>[2x]MRRETVGEFSSDDDDDILLELGTRPPRFTQIPPSSAALQTQIPTTLEVTTTTLNNKQSKNDNQLVNQLNKAQGEASMLRDKINFLNIEREKEKNIQAVKVNELQVKHLQELAKLKQELQKLEDEKKFLQMEARGKSKREVITNVKPPSTTLSTNTNTITPDSSSVAIEAKPQSPQSKKRKISDNLLKKNMVPLNPNRIIPDETSLFLESILLHQIIGADLSTIEILNRLKLDYITEFKFKNFVIAKGAPIGKSIVSLLLRCKKTLTLDRFIDTLLEDIAVLIKEISVHPNESKLAVPFLVALMYQIVQFRPSATHNLALKDCFLFICDLIRIYHHVLKVPIHESNMNLHVEPQIFQYELIDYLIISYSFDLLEGILRVLQSHPKQTYMEFFDENILKSFEFVYKLALTISYKPMVNVIFSAVEVVNIITSIILNMDNSSDLKSLISGSWWRDCITRLYALLEKEIKSGDVYNENVDTTTLHMSKYHDFFGLIRNIGDNELGGLISKLIYTDRLQSVPRVISKEDIGMDSDKFTAPIIGYKMEKWLLKLKDEVLNIFENLLMIYGDDATIVNGEMLIHSSKFLSREQALMIERYVGQDSPNLDLRCHLIEHTLTIIYRLWKDHFKQLREEQIKQVESQLIMSLWRFLVCQTETVTANEREMRDHRHLVDSLHDLTIKDQASYYEDAFEDLPEYIEEELKMQLNKRTGRIMQVKYDEKFQEMARTILESKSFDLTTLEEADSLYISMGL;>[2x]MESHVKYLDELILAIKDLNSGVDSKVQIKKVPTDPSSSQEYAKSLKILNTLIRNLKDQRRNNIMKNDTIFSKTVSALALLLEYNPFLLVMKDSNGNFEIQRLIDDFLNISVLNYDNYHRIWFMRRKLGSWCKACVEFYGKPAKFQLTAHFENTMNLYEQALTEVLLGKTELLKFYDTLKGLYILLYWFTSEYSTFGNSIAFLDSSLGFTKFDFNFQRLIRIVLYVFDSCELAALEYAEIQLKYISLVVDYVCNRTISTALDAPALVCCEQLKFVLTTMHHFLDNKYGLLDNDPTMAKGILRLYSLCISNDFSKCFVDHFPIDQWADFSQSEHFPFTQLTNKALSIVYFDLKRRSLPVEALKYDNKFNIWVYQSEPDSSLKNVTSPFDDRYKQLEKLRLLVLKKFNKTERGTLLKYRVNQLSPGFFQRAG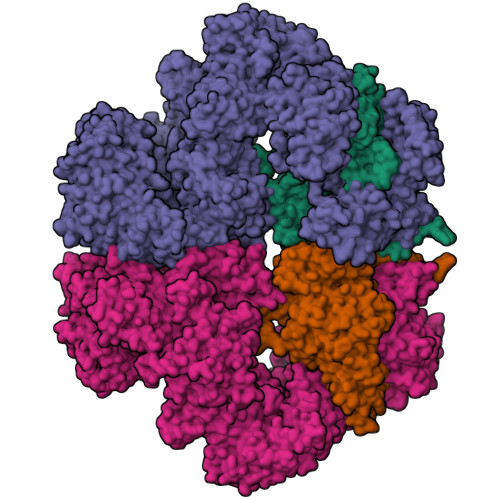NDFKLILNEASVSIQTCFKTNNITRLTSWTVILGRLACLESEKFSGTLPNSTKDMDNWYVCHLCDIEKTGNPFVRINPNRPEAAGKSEIFRILHSNFLSHPNIDEFSESLLSGILFSLHRIFSHFQPPKLTDGNGQINKSFKLVQKCFMNSNRYLRLLSTRIIPLFNISDSHNSEDEHTATLIKFLQSQKLPVVKENLVIAWTQLTLTTSNDVFDTLLLKLIDIFNSDDYSLRIMMTLQIKNMAKILKKTPYQLLSPILPVLLRQLGKNLVERKVGFQNLIELLGYSSKTILDIFQRYIIPYAIIQYKSDVLSEIAKIMCDGDTSLINQMKVNLLKKNSRQIFAVALVKHGLFSLDILETLFLNRAPTFDKGYITAYLPDYKTLAEITKLYKNSVTKDASDSENANMILCSLRFLITNFEKDKRHGSKYKNINNWTDDQEQAFQKKLQDNILGIFQVFSSDIHDVEGRTTYYEKLRVINGISFLIIYAPKKSIISALAQISICLQTGLGLKEVRYEAFRCWHLLVRHLNDEELSTVIDSLIAFILQKWSEFNGKLRNIVYSILDTLIKEKSDLILKLKPYTTLALVGKPELGILARDGQFARMVNKIRSTTDLIPIFANNLKSSNKYVINQNLDDIEVYLRRKQTERSIDFTPKKVGQTSDITLVLGALLDTSHKFRNLDKDLCEKCAKCISMIGVLDVTKHEFKRTTYSENEVYDLNDSVQTIKFLIWVINDILVPAFWQSENPSKQLFVALVIQESLKYCGLSSESWDMNHKELYPNEAKLWEKFNSVSKTTIYPLLSSLYLAQSWKEYVPLKYPSNNFKEGYKIWVKRFTLDLLKTGTTENHPLHVFSSLIREDDGSLSNFLLPYISLDIIIKAEKGTPYADILNGIIIEFDSIFTCNLEGMNNLQVDSLRMCYESIFRVFEYCKKWATEFKQNYSKLHGTFIIKDTKTTNMLLRIDEFLRTTPSDLLAQRSLETDSFERSALYLEQCYRQNPHDKNQNGQLLKNLQITYEEIGDIDSLDGVLRTFATGNLVSKIEELQYSENWKLAQDCFNVLGKFSDDPKTTTRMLKSMYDHQLYSQIISNSSFHSSDGKISLSPDVKEWYSIGLEAANLEGNVQTLKNWVEQIESLRNIDDREVLLQYNIAKALIAISNEDPLRTQKYIHNSFRLIGTNFITSSKETTLLKKQNLLMKLHSLYDLSFLSSAKDKFEYKSNTTILDYRMERIGADFVPNHYILSMRKSFDQLKMNEQADADLGKTFFTLAQLARNNARLDIASESLMHCLERRLPQAELEFAEILWKQGENDRALKIVQEIHEKYQENSSVNARDRAAVLLKFTEWLDLSNNSASEQIIKQYQDIFQIDSKWDKPYYSIGLYYSRLLERKKAEGYITNGRFEYRAISYFLLAFEKNTAKVRENLPKVITFWLDIAAASISEAPGNRKEMLSKATEDICSHVEEALQHCPTYIWYFVLTQLLSRLLHSHQSSAQIIMHILLSLAVEYPSHILWYITALVNSNSSKRVLRGKHILEKYRQHSQNPHDLVSSALDLTKALTRVCLQDVKSITSRSGKSLEKDFKFDMNVAPSAMVVPVRKNLDIISPLESNSMRGYQPFRPVVSIIRFGSSYKVFSSLKKPKQLNIIGSDGNIYGIMCKKEDVRQDNQYMQFATTMDFLLSKDIASRKRSLGINIYSVLSLREDCGILEMVPNVVTLRSILSTKYESLKIKYSLKSLHDRWQHTAVDGKLEFYMEQVDKFPPILYQWFLENFPDPINWFNARNTYARSYAVMAMVGHILGLGDRHCENILLDIQTGKVLHVDLDCLFEKGKRLPVPEIVPFRLTPNLLDALGIIGTEGTFKKSSEVTLALMRKNEVALMNVIETIMYDRNMDHSIQKALKVLRNKIRGIDPQDGLVLSVAGQTETLIQEATSEDNLSKMYIGWLPFW> IKKIPMIIGGAERDTSEHEYRELTLNSYKVSIPIINQDDVEAIKSQSVENNLNINQIVNFLYTVGQKWKSENYSRRLTYIRDLVRFLGYSPEMAKLEANWISMILSSKSALYDIVETELGSRHIVDEWLPQGDCYVKAMPKGKSVHLLAGNVPLSGVTSIIRAILTKNECIIKTSSADPFTAIALASSFIDTDEHHPISRSMSVMYWSHNEDIAIPQQIMNCADVVVSWGGY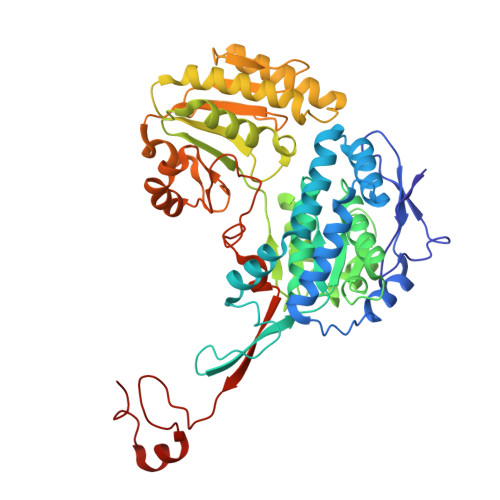DAIKWATEHTPVNVDILKFGPKKSIAIVDNPVDITASAIGVAHDICFYDQQACFSTQDIYYIGDNIDAFFDELVEQLNLYMDILPKGDQTFDEKASFSLIEKECQFAKYKVEKGDNQSWLLVKSPLGSFGNQPLARSAYIHHVSDISEITPYIENRITQTVTVTPWESSFKYRDVLASHGAERIVESGMNNIFRVGGAHDGMRPLQRLVKYISHERPYTYSTKDVAVKIEQTRYLEEDKFLVFVP> MAVERTLII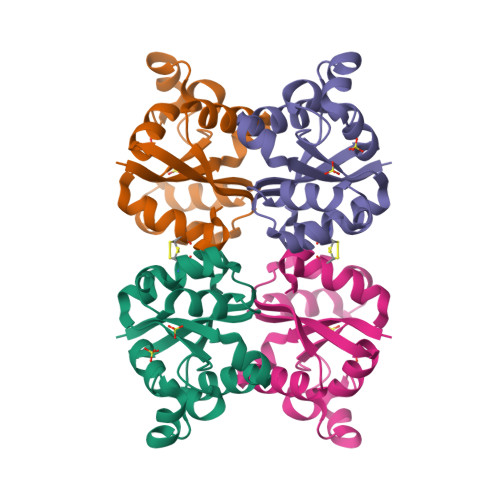VKPDAMEKGALGKILDRFIQEGFQIKALKMFRFTPEKAGEFYYVHRERPFFQELVEFMSSGPVVAAVLEGEDAIKRVREIIGPTDSEEARKVAPNSIRAQFGTDKGKNAIHASDSPESAQYEICFIFSGLEIV> MNQNLLVTKRDGSTERINLDKIHRVLDWAAEGLHNVSISQVELRSHIQFYDGIKTSDIHETIIKAAADLIS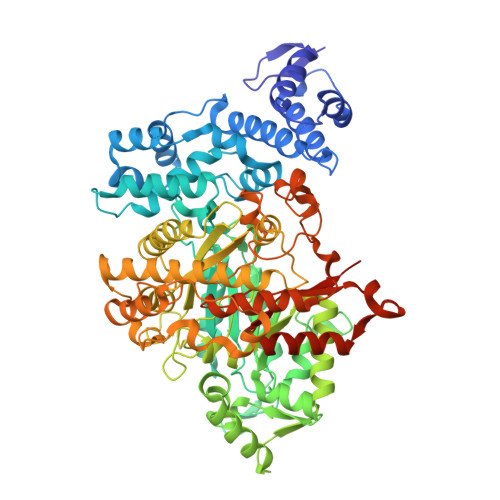RDAPDYQYLAARLAIFHLRKKAYGQFEPPALYDHVVKMVEMGKYDNHLLEDYTEEEFKQMDTFIDHDRDMTFSYAAVKQLEGKYLVQNRVTGEIYESAQFLYILVAACLFSNYPRETRLQYVKRFYDAVSTFKISLPTPIMSGVRTPTRQFSSCVLIECGDSLDSINATSSAIVKYVSQRAGIGINAGRIRALGSPIRGGEAFHTGCIPFYKHFQTAVKSCSQGGVRGGAATLFYPMWHLEVESLLVLKNNRGVEGNRVRHMDYGVQINKLMYTRLLKGEDITLFSPSDVPGLYDAFFADQEEFERLYTKYEKDDSIRKQRVKAVELFSLMMQERASTGRIYIQNVDHCNTHSPFDPAIAPVRQSNLCLEIALPTKPLNDVNDENGEIALCTLSAFNLGAINNLDELEELAILAVRALDALLDYQDYPIPAAKRGAMGRRTLGIGVINFAYYLAKHGKRYSDGSANNLTHKTFEAIQYYLLKASNELAKEQGACPWFNETTYAKGILPIDTYKKDLDTIANEPLHYDWEALRESIKTHGLRNSTLSALMPSETSSQISNATNGIEPPRGYVSIKASKDGILRQVVPDYEHLHDAYELLWEMPGNDGYLQLVGIMQKFIDQSISANTNYDPSRFPSGKVPMQQLLKDLLTAYKFGVKTLYYQNTRDGAEDAQDDLVPSIQDDGCESGACKI>[2x]MGSSHHHHHHGSGGGNNNNNNNNNNLGIEENLYFQSHMMKFTVEREHLLKPLQQVSGPLGGRPTLPILGNLLLQVADGTLSLTGTDLEMEMVARVALVQPHEPGATTVPARKFFDICRGLPEGAEIAVQLEGERMLVRSGRSRFSLSTLPAADFPNLDDWQSEVEFTLPQATMKRLIEATQFSMAHQDVRYYLNGMLFETEGEELRTVATDGHRLAVCSMPIGQSLPSHSVIVPRKGVIELMRMLDGGDNPLRVQIGSNNIRAHVGDFIFTSKLVDGRFPDYRRVLPKNPDKHLEAGCDLLKQAFARAAILSNEKFRGVRLYVSENQLKITANNPEQEEAEEILDVTYSGAEMEIGFNVSYVLDVLNALKCENVRMMLTDSVSSVQIEDAASQSAAYVVMPMRLVDSGASGGSWLRQAQLT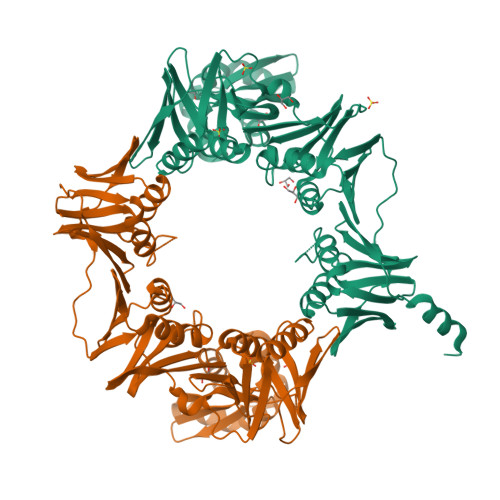PGEAPVCAQPLLIPLRLKVSAEEKSALEKAQSALAELGIDFQSDAQHVTIRAVPLPLRQQNLQILIPELIGYLAKQSVFEPGNIAQWIARNLMSEH> GPLGSQRKEKDFQGMLEYHKEDEALLIRNLVTDLKPQMLSGTVPCLPAYILYMCIRHADYTNDDLKVHSLLTSTINGIKKVLKKHNDDFEMTSFWLSNTCRLLHCLKQYSGDEGFMTQNTAKQNEHCLKNFDLTEYRQVLSDLSIQIYQQLIKIAEGVLQPMIVSAMLENESIQGLSGVKPTGYRKRSSSMADGDNSYCLEAIIRQMNAFHTVMCDQGLDPEIILQVFKQLFYMINAVTLNNLLLRKDVCSWSTGMQLRYNISQLEEWLRGRNLHQSGAVQTMEPLIQAAQLLQLKKKTQEDAEAICSLCTSLSTQQIVKILNLYTPLNEFEERVTVAFIRTIQAQLQERNDPQQLLLDAKHMFPVLFPFNPSSLTMDSIHIPACLNLEFLNEV

Type V myosin (MyoV) motors move protein complexes, organelles, vesicles, and mRNAs along actin cables. The C-terminal globular domain (GD) defines this class of myosins and mediates the majority of cargo interactions. In vertebrate Myo5a, the GD also mediates autoinhibition of ATPase activity in its cargo-free state. In this study, we describe the high-resolution X-ray structures of the GDs from human Myo5a and Myo5b as well as low-resolution SAXS-surface envelopes for all three human MyoV paralogs.

The structure of Myo5b GD was solved at 3.1 Å resolution by molecular replacement using Myo5a GD as template. The asymmetric unit contains one Myo5b molecule (Rwork = 0.25, Rfree = 0.31), which shares with Myo5a the overall conservation of domain organization. An overlay of both structures reveals a root mean square deviation (RMSD) of only 1.1 Å. No electron density was visible for the N-terminal four amino acids, for loop I from amino acids 1625 to 1651 and for loop II (1781 to 1789). Myo5a and Myo5b GDs share 70.5% identical amino acids. A higher degree of deviation was observed for Myo5b. However, these two residues are fully conserved in all three paralogs (red-boxed amino acids) and are in the same position in Myo5a, Myo5b, and Myo5c. This observation suggests that autoinhibition might not be limited to Myo5a.>GSHMESFLLSKVSFVIKKIRLEKGMTQEDLAYKSNLDR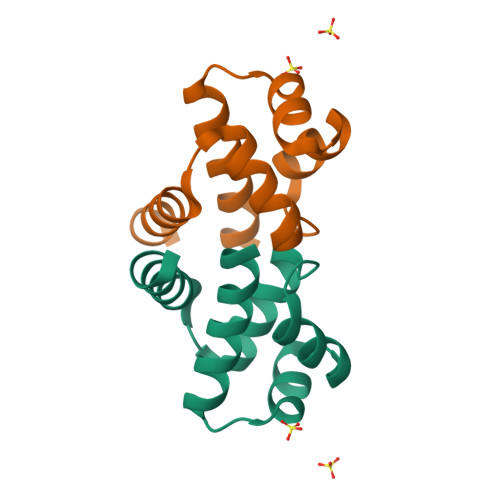TYISGIERNSRNLTIKALELIMKGLEVSDVVFFEMLIKEILKHD[2x]>GHMETGDQRFGDLVFRQLAPNVWQHTSYLDMPGFGAVAPSNGLIVRDGGRVLVVDTAWTDDQTAQILNWIKQEINLPVALAVVTHAHQDKMGGMDALHAAGIATYANALSNQLAPQEGMVAAQHSLT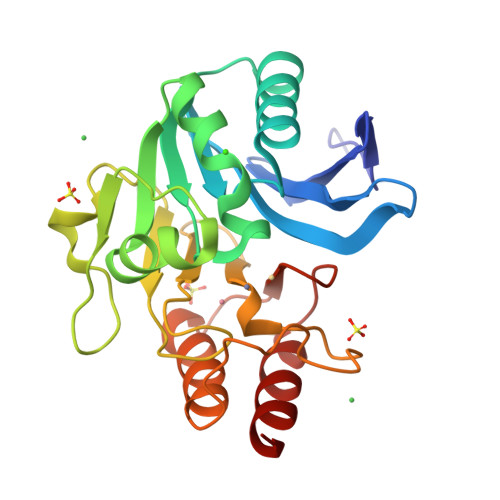FAANGWVEPATAPNFGPLKVFYPGPGHTSDNITVGIDGTDIAFGGCLIKDSKAKSLGNLGDADTEHYAASARAFGAAFPKASMIVMSHSAPDSRAAITHTARMADKLR[4x]>[3x]SGNFCPLCDKCYDDDDYESK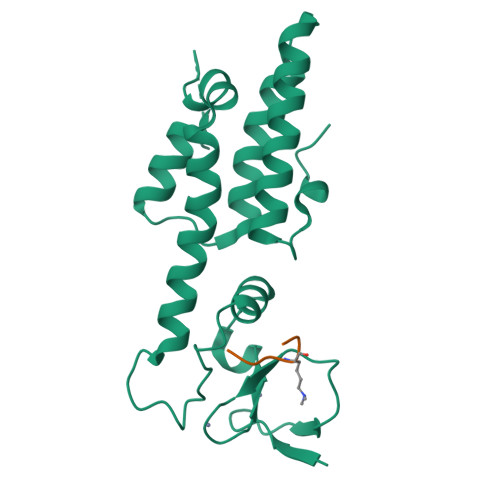MMQCGKCDRWVHSKCENLSDEMYEILSNLPESVAYTCVNCTERHPAEWRLALEKELQISLKQVLTALLNSRTTSHLLRYRQQQPLDLEGVKRKMDQGNYTSVLEFSDDIVKIIQAAINSDGGQPEIKKANSMVKSFFIRQMERVFPWFSVKKSRFWEPNKVSS;>ARTKQTARK[3x]Vps34, the primordial phosphatidylinositol 3-kinase (PtdIns3K) that phosphorylates the 3-OH of phosphatidylinositol to form phosphatidylinositol 3-phosphate (PtdIns3P), is conserved in all eukaryotes, and it is important both for endocytic traffic to lysosomes and vacuoles and for autophagy. The minimal Vps34 complex is a heterodimer of Vps34 with Vps15, a putative protein kinase. This Vps34-Vps15 complex is the core for 2 larger, heterotetrameric assemblies known as complexes I and II. In addition to the Vps34-Vps15 core, complex I includes an accessory pair of proteins, Vps30/Atg6 (BECN1 in mammals) and Atg14 (ATG14 in mammals).

We determined a 28-Å resolution structure of the isolated Vps15-Vps34 heterodimer, which suggests that the structure of this heterodimeric core is similar to what is observed in complex II that does not bind Atg38. The low-resolution EM structure of the yeast Vps15-Vps34 subcomplex shows that the 2 components formed a stable core, and this assembly may also exist in mammalian cells.

> MGAQLSLVVQASPSIAIFSYIDVLEEVHYVSQLNSSRFLKTCKALDPNGEIVIKVFIKPKDQYSLRPFLQRIRAQSFKLGQLPHVLNYSKLIETNRAGYMIRQHLKNNLYDRLSLRPYLQDIELKFIAFQLLNALKDIHNLNIVHGDIKTENILVTSWNWCILTDFAAFIKPVYLPEDNPGEFLFYFDTSKRRTCYLAPERFNSKLYQDGKSNNGRLTKEMDIFSLGCVIAEIFAEGRPIFNLSQLFKYKSNSYDVNREFLMEEMNSTDLRNLVLDMIQLDPSKRLSCDELLNKYRGIFFPDYFYTFIYDYFRNLVTMTTSTPISDNTCTNSTLEDNVKLLDETTEKIYRDFSQICHCLDFPLIKDGGEIGSDPPILESYKIEIEISRFLNTNLYFPQNYHLVLQQFTKVSEKIKSVKEECALLFISYLSHSIRSIVSTATKLKNLELLAVFAQFVSDENKIDRVVPYFVCCFEDSDQDVQALSLLTLIQVLTSVRKLNQLNENIFVDYLLPRLKRLLISNRQNTNYLRIVFANCLSDLAIIINRFQEFTFAQHCNDNSMDNNTEIMESSTKYSAKLIQSVEDLTVSFLTDNDTYVKMALLQNILPLCKFFGRERTNDIILSHLITYLNDKDPALRVSLIQTISGISILLGTVTLEQYILPLLIQTITDSEELVVISVLQSLKSLFKTGLIRKKYYIDISKTTSPLLLHPNNWIRQFTLMIIIEIINKLSKAEVYCILYPIIRPFFEFDVEFNFKSMISCCKQPVSRSVYNLLCSWSVRASKSLFWKKIITNHVDSFGNNRIEFITKNYSSKNYGFNKRDTKSSSSLKGIKTSSTVYSHDNKEIPLTAEDRNWIDKFHIIGLTEKDIWKIVALRGYVIRTARVMAANPDFPYNNSNYRPLVQNSPPNLNLTNIMPRNIFFDVEFAEESTSEGQDSNLENQQIYKYDESEKDSNKLNINGSKQLSTVMDINGSLIFKNKSIATTTSNLKNVFVQLEPTSYHMHSPNHGLKDNANVKPERKVVVSNSYEGDVESIEKFLSTFKILPPLRDYKEFGPIQEIVRSPNMGNLRGKLIATLMENEPNSITSSAVSPGETPYLITGSDQGVIKIWNLKEIIVGEVYSSSLTYDCSSTVTQITMIPNFDAFAVSSKDGQIIVLKVNHYQQESEVKFLNCECIRKINLKNFGKNEYAVRMRAFVNEEKSLLVALTNLSRVIIFDIRTLERLQIIENSPRHGAVSSICIDEECCVLILGTTRGIIDIWDIRFNVLIRSWSFGDHAPITHVEVCQFYGKNSVIVVGGSSKTFLTIWNFVKGHCQYAFINSDEQPSMEHFLPIEKGLEELNFCGIRSLNALSTISVSNDKILLTDEATSSIVMFSLNELSSSKAVISPSRFSDVFIPTQVTANLTMLLRKMKRTSTHSVDDSLYHHDIINSISTCEVDETPLLVACDNSGLIGIFQ;> MSLNNITFCVSQDLDVPLKVKIKSLEGHKPLLKPSQKILNPELMLIGSNVFPSSDLIVSLQVFDKERNRNLTLPIYTPYIPFRNSRTWDYWLTLPIRIKQLTFSSHLRIILWEYNGSKQIPFFNLETSIFNLKDCTLKRGFESLKFRYDVIDHCEVVTDNKDQENLNKYFQGEFTRLPWLDEITISKLRKQRENRTWPQGTFVLNLEFPMLELPVVFIEREIMNTQMNIPTLKNNPGLSTDLREPNRNDPQIKISLGDKYHSTLKFYDPDQPNNDPIEEKYRRLERASKNANLDKQVKPDIKKRDYLNKIINYPPGTKLTAHEKGSIWKYRYYLMNNKKALTKLLQSTNLREESERVEVLELMDSWAEIDIDDALELLGSTFKNLSVRSYAVNRLKKASDKELELYLLQLVEAVCFENLSTFSDKSNSEFTIVDAVSSQKLSGDSMLLSTSHANQKLLKSISSESETSGTESLPIVISPLAEFLIRRALVNPRLGSFFYWYLKSESEDKPYLDQILSSFWSRLDKKSRNILNDQVRLINVLRECCETIKRLKDTTAKKMELLVHLLETKVRPLVKVRPIALPLDPDVLICDVCPETSKVFKSSLSPLKITFKTTLNQPYHLMFKVGDDLRQDQLVVQIISLMNELLKNENVDLKLTPYKILATGPQEGAIEFIPNDTLASILSKYHGILGYLKLHYPDENATLGVQGWVLDNFVKSCAGYCVITYILGVGDRHLDNLLVTPDGHFFHADFGYILGQDPKPFPPLMKLPPQIIEAFGGAESSNYDKFRSYCFVAYSILRRNAGLILNLFELMKTSNIPDIRIDPNGAILRVRERFNLNMSEEDATVHFQNLINDSVNALLPIVIDHLHNLAQYWRT Enzymes in the Gcn5-related N-acetyltransferase (GNAT) superfamily are widespread and critically involved in multiple cellular processes ranging from antibiotic resistance to histone modification. Previously, we determined the structure of the PA3944 GNAT enzyme from Pseudomonas aeruginosa and found that it could acetylate polymyxin antibiotics, specifically the 3-Dab residue on polymyxin B and on colistin. The canonical chemical mechanism attributed to GNATs is a general acid/base mechanism; however, mounting evidence has cast doubt on the applicability of this mechanism to all GNATs. This study shows that the Pseudomonas aeruginosa PA3944 enzyme uses a nucleophilic serine residue and a hybrid ping-pong mechanism for catalysis instead of a general acid/base mechanism. Instead, PA3944 has a serine (S148) in a comparable location as the typical critical tyrosine residue found in GNATs.

Since our kinetic studies showed the enzyme utilized a ping-pong or hybrid ping-pong mechanism, we attempted to obtain a crystal structure of the protein with S148 acetylated. All of our previous structures of the enzyme were determined in the presence of CoA. Therefore, we co-crystallized the protein in the presence of AcCoA and looked for density around S148 for an acetyl group. In addition to adding AcCoA for co-crystallization, we also included (R)-3-(2-chloroacetamido)-4-(((S)-1-methoxy-1-oxo-3-phenylpropan-2-yl)amino)-4-oxobutanoic acid. While this compound was present in the crystallization solution, it was not observed in the crystal structure; the rationale and synthesis of this compound as an alternate substrate will be described in a separate manuscript. In the presence of these compounds, the enzyme also crystallized in the P1 space group with two molecules in the asymmetric unit. Based on the observed electron density, we modeled CoA in chain A and AcCoA in chain B. In this structure, we did not observe any additional density around S148 that would indicate its acetylation in the crystal. However, we did observe a very small amount of AcCoA cleavage in the presence of the enzyme and absence of acceptor substrates in our kinetic assays, possibly indicating the enzyme could form an acyl-enzyme intermediate required for a kinetic mechanism with a ping-pong component. Further studies are necessary to show the acyl-enzyme intermediate is indeed formed but are beyond the scope of this current study. This structure was nonetheless useful for docking experiments. Therefore, we first docked NANMO into the WT structure with AcCoA to determine which residues might interact with the protonated and free base forms of the molecule.

>[2x]GHMNANLPPSAISELHGPRLLLRAWRDSDREAFAEMCADPQVMEFFPSVLDRAQSDALVDRVQAHFAERGYGPWALELPGEAAFIGFTGLFDVTMDVHFAPTVEIGWRLAPAYWGRGLAREAAETALDFAFERLRLPEVVAFTTPPNRRSWGLMERLGMRRDPAEDFDHPLLAADHPMRRHILYRVDAARWAER The pyruvate dehydrogenase complex (PDC) is a central metabolic enzyme in all living cells composed majorly of E1, E2, and E3. The 2-oxoacid dehydrogenase complexes are a class of protein complexes with acyl-transferase activity in metabolism and amino acid synthesis. They co-localize 3 catalytic components (E1-3) that act in sequence upon a substrate-carrying lipoyl domain(LD) that is flexibly linked to E2. Like mammals, fungi also utilize E3BP to recruit E321,23–25. The cryo-EM reconstruction of the CBD from N.crassa E3BP inside the PDC core here reveals its oligomeric form and specific interactions.

CBD-occupied E2-trimers were selected by classification, and mapped back to the cores particles from which they were extracted, which permitted analysis of how many CBD trimers were found within each core particle. The majority of E2 core particles had 3-4 CBD trimers assigned, whereas only 4% were assigned 5 or more CBD-trimers. The analysis was repeated using native PDC data EMPIAR-1048929, which found a highly similar CBD-trimer distribution. Increased uncertainty in both classified proportions and attained were however noted due to the higher overall noise in this data, to the extent that it can only quantifiably corroborate the existence and predominance of the CBD trimer in native samples compared to the recombinant expression, and conversely cannot confirm specific interactions observed in the latter. The CBD of N.crassa has a trimeric interface with a symmetry axis that coincides with that of a core E2 CTD-trimer. Additionally, the trimeric form of N.crassa CBD provides a steric limit to 12 bound copies of E3BP per core assembly.

>[6x]MIVPVLSRQALRHASVARVALPSLTRWYASYPPHTVVKMPALSPTMTSGGIGAWQKKPGDKIEPGEVLVEIETDKAQMDFEFQEEGVLAKILKDSGEKDVAVGNPIAILVEEGTDVNAFKDFTLKDAGGETSPAVPKDEPKNESTASAPTPAPTPAPEPENTSFTGRFQTALEREPNALPAAKRLAREKGIDLRNVKGSGPGGKITEEDVKKALASAPAAGAAAAAYTDVPISGMRKTIAARLKESVTENPHFFVSTNLSVSKLLKLRQALNSSADGRYKLSVNDFLIKAMGIASKRVPTVNSSWRDGVIRQFETVDVSVAVATPNGLITPIVKGVEGKGLESISAAVKELAKKARDGKLKPEEYQGGSISISNMGMNPAVQSFTAIINPPQAAILAVGAPQKVAVPVENEDGTTGVSWDEQIIVTASFDHKVVDGAVGAEWIRELKKVIENPLELLL;>MASLTAACRISARMAGRSVRGFRTSAAALAAQNFTMPALSPTMTEGNIATWRVKEGDKFSAGDVLLEIETDKATMDVEAQDDGVMVKIMKNDGAKGVAVGARIAVIAEEGDDISSLEIPADAAPQSKPAESAPSAPPPPTTADQSNVAVPESAPQNASSKSAPKPPKRQYPHYPSVAHLLKVNGIDAAAVKDITPTGPGGRLLKGDVLAYLGKINAQTPSTVSERFEKQSHLDLSNIKVAKSTEAVKATTEKAQSKKLDAPAPPPVAVVTAPISLSAAIDVQNKLHKTIGVFLPLSTFITRATEIANQKLPLPANYQPTADELFNQVLGLDKVTRKESRGSYTPTFGSFVAPQRAARKADIIDILAAPSTRVAASAQSKSAAPGLTTSGPNVFSLQVPKSEEKRAQAFLQKMKLVLEQEPDKLVRA[3x]> AAVQELSIERLLEMESLVADPSEEFQFLRVGPDSNVPPKFRAPVSSLCQIGNKQIAALVVWARDIPHFSQLEMEDQILLIKGSWNELLLFAIAWRSMEFLTEERDGVDGTGNRTTSPPQLMCLMPGMTLHRNSALQAGVGQIFDRVLSELSLKMRTLRVDQAEYVALKAIILLNPDVKGLKNRQEVE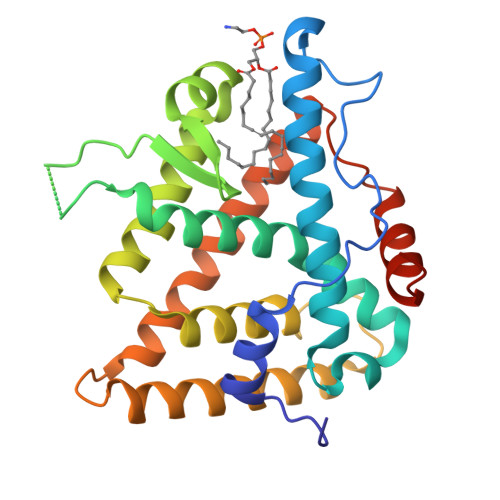VLREKMFLCLDEYCRRSRSSEEGRFAALLLRLPALRSISLKSFEHLFFFHLVADTSIAGYIRDALRNHAPPIDTNMM6-amino-5-fluorouridine 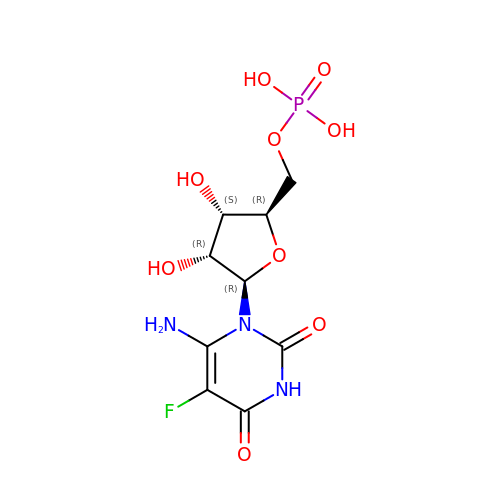5'-(dihydrogen phosphate) | C9 H13 F N3 O9 P | OLBMCLUPWOAIRA-UMMCILCDSA-N>[2x]GPHMLEAEHPLQYNYTFWYSRRTPGRPTSSQSYEQNIKQIGTFASVEQFWRFYSHMVRPGDLTGHSDFHLFKEGIKPMWEDDANKNGGKWIIRLRKGLASRCWENLIL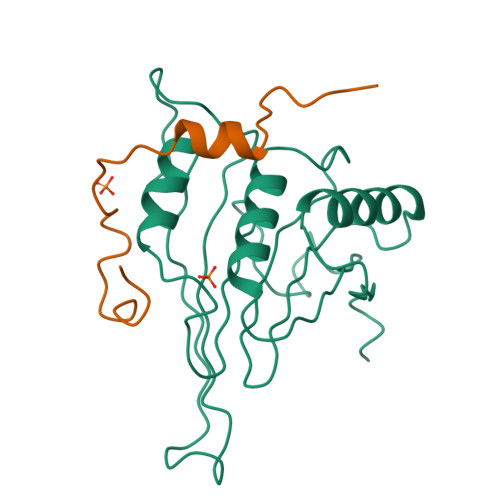AMLGEQFMVGEEICGAVVSVRFQEDIISIWNKTASDQATTARIRDTLRRVLNLPPNTIMEYKTHTDSIKMPGRLGPQRLLF;>[2x]GPHMKYKLADYRYGREEMLALFLKDNKIPSDLLDKEFLPILQ S-P-NITROBENZYLOXYCARBONYLGLUTATHIONE | C18 H24 N4 O10 S | 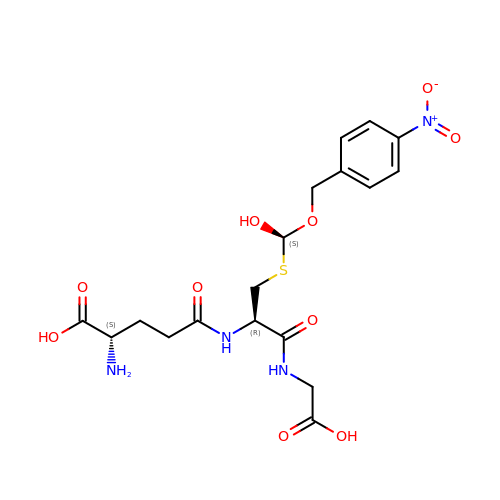QYFGPQQSJQOGEO-TVJRNMROSA-N> PSSSMADFRKFFAKAKHIVIISGAGVSAESGVPTFRGAGGYWRKWQAQDLATPLAFAHNPSRVWEFYHYRREVMGSKEPNAGHRAIAECETRLGKQGRRVVVITQNIDELHRKAGTKNLLEIHGSLFKTRCTSCGVVAENYKSPICPALSGKGAPEPGTQDASIPVEKLPRCEEAGCGGLLRPHVVWFGENLDPAILEEVDRELAHCDLCLVVGTSSVVYPAAMFAPQVAARGVPVAEFNTETTPATNRFRFHFQGPCGTTLPEALA;> Y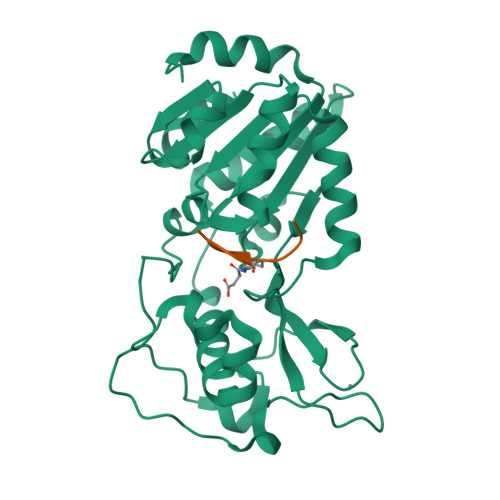ALXRQG> QSTQIKIERDNYGVPHIYANDTYSLFYGYGYAVAQ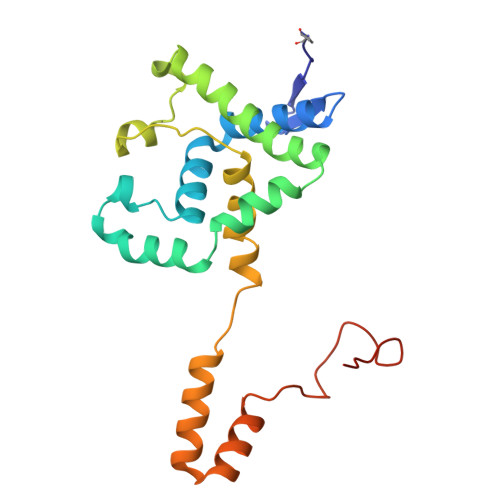DRLFQMEMAKRSTQGTVSEVFGKDYISFDKEIRNNYWPDSIHKQINQLPSQEQDILRGYADGMNAWIKQINTKPDDLMPKQFIDYDFLPSQWTSFDVAMIMVGTLANRFSDMNSEIDNLALLTALKDKYGEQLGVEFFNQINWLNNPNAPTTISSEEFTYSDSQKTKNIS>[5x]GMSNINYVILTVASVDFSYRETMARLMSSYSKDLIDNAGAKGTRFGSIGTGDHAGSLIFIQFYDDLTGYQKALEIQSKSSV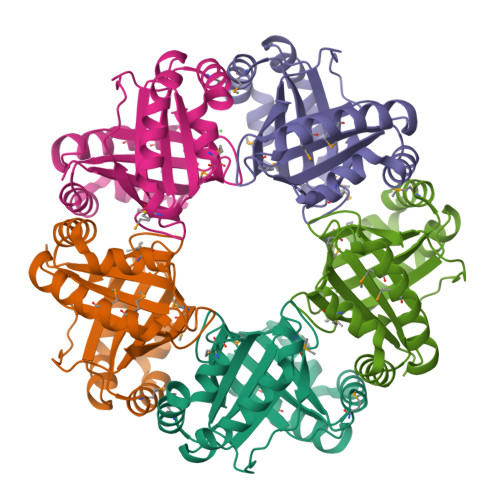FKEIMDSGKANIYLRNISTSLPTKFEQSYEHPKYIVLTRAEAAMSDKDKFLNCINDTASCFKDNGALTLRFGNLLTGSNVGNYLLGVGYPSMEAIEKTYDELLAHSSYKELMTFAKVNMRNIIKIL> DEDKW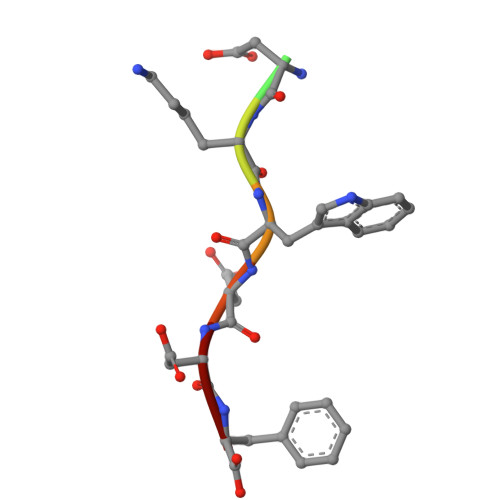DDF>MRSRRVDVMDVMNRLILAMDLMNRDDALRVTGEVREYIDTVKIGYPLVLSEGMDIIAEFRKRFGCRIIADFKVADIPETNEKICRATFKAGADAIIVHGFPGADSVRACLNVAEEMGREVFLLTEMSHPGAEMFIQGAADE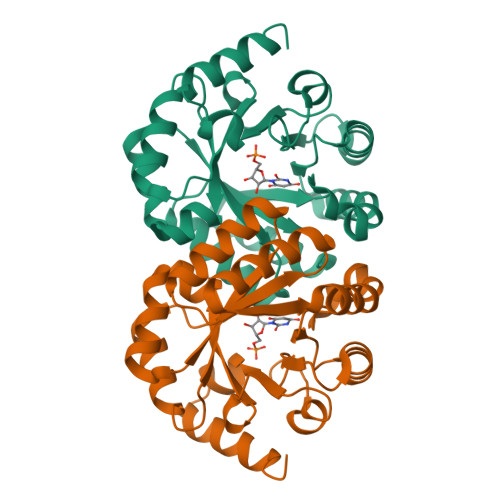IARMGVDLGVKNYVGPSTRPERLSRLREIIGQDSFLISPGVGAQGGDPGETLRFADAIIFGRSIYLADNPAAAAAGIIESIKDLLNP[2x]> MSALFEPYTLKDVTLRNRIAIPPMSQYMAEDGMINDWHHVHLAGLARGGAGLLVVEATAVAPEGRITPGCAGIWSDAHAQAFVPVVQAIKAAGSVPGIQIAHAGRKASANRPWEGDDHIAADDTRGWETIAPSAIAFGAHLPKVPREMTLDDIARVKQDFVDAARRARDAG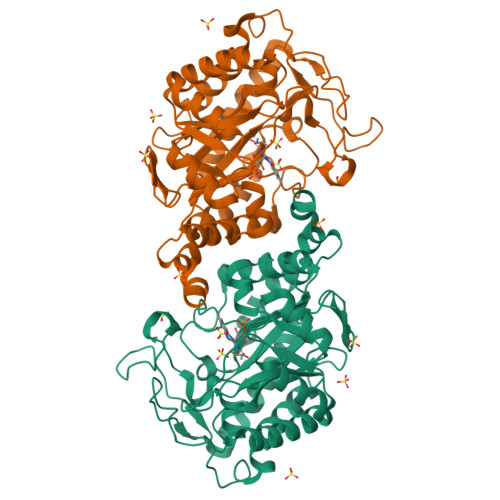FEWIELHFAHGYLGQSFFSEHSNKRTDAYGGSFDNRSRFLLETLAAVREVWPENLPLTARFGVLEYDGRDEQTLEESIELARRFKAGGLDLLSVSVGFTIPDTNIPWGPAFMGPIAERVRREAKLPVTSAWGFGTPQLAEAALQANQLDLVSVGRAHLADPHWAYFAAKELGVEKASWTLPAPYAHWLERYR>GSAKDPSADQANADKVMTKDLEIDRATREVIFKGDLITLTRTEFDLLLFLASNLGRVFTRDELLDHVWGYNHFPTTRTVDTHVLQLRQKLPGLEIETLRGV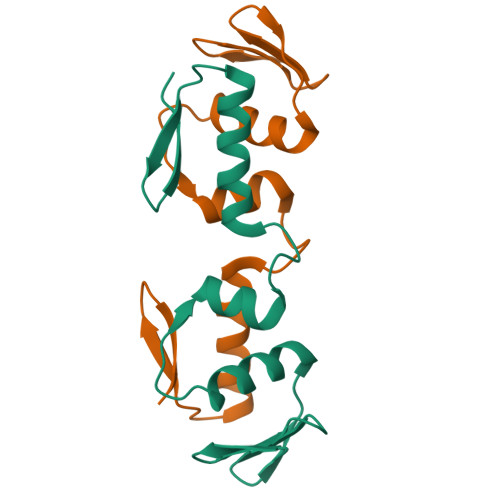GYKMKA[2x]> GPTHRFVQKVEEMVQNHMTYSLQDVGGDANWQLVVEEGEMKVYRREVEENGIVLDPLKATHAVKGVTGHEVCNYFWNVDVRNDWETTIENFHVVETLADNAIIIYQTHKRVWPASQRDVLYLSVIRKIPALTENDPETWIVCNFSVDHDSAPLNNRCVRAKINVAMICQTLVSPPEGNQEISRDNILCKITYVANVNPGGWAPASVLRAVAKREYPKFLKRFTSYVQEKTAGKPI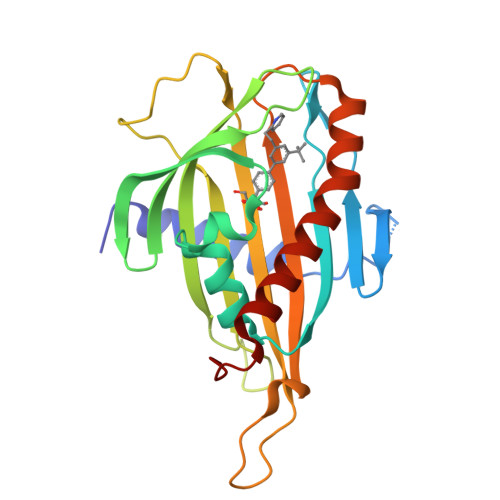LF> SFTMSGGFELQPRDGGPRVALAPGETVIGRGPLLGITDKRVSRRHAILEVAGGQLRIKPIHTNPCFYQSSEKSQLLPLK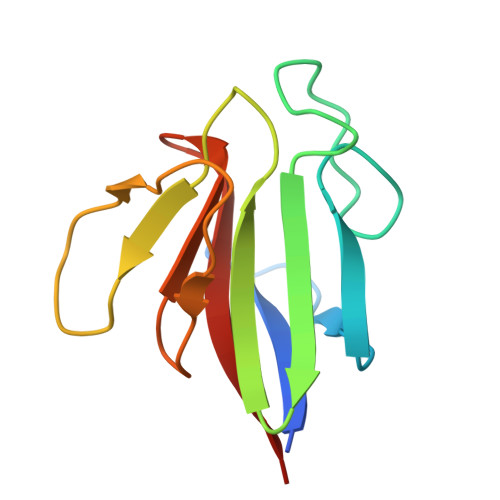PNLWCYLNPGDSFSLLVDKYIFRILSIPS>[3x]NAMLASEVIQAYEAFCPQEFSMEGDSRGLQIGTLDKGIQRVMVALDIREETV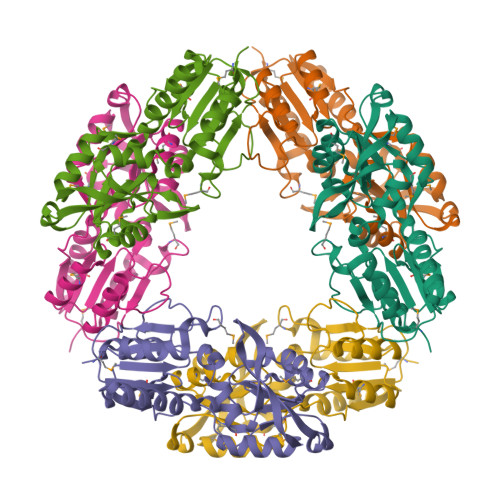AEAIEKGVDLIIVKHAPIFRPIKDLLASRPQNQIYIDLIKHDIAVYVSHTNIDIVENGLNDWFCQMLGIEETTYLQETGPERGIGRIGNIQPQTFWELAQQVKQVFDLDSLRMVHYQEDDLQKPISRVAICGGSGQSFYKDALAKGADVYITGDIYYHTAQDMLSDGLLALDPGHYIEVIFVEKIAALLSQWKEDKGWSIDILPSQASTNPFHHI Here, an automated procedure is described to identify the positions of many cryocooled crystals mounted on the same sample holder, to rapidly predict and rank their relative diffraction strengths and to collect partial X-ray diffraction data sets from as many of the crystals as desired. Subsequent hierarchical cluster analysis then allows the best combination of partial data sets, optimizing the quality of the final data set obtained. To demonstrate the general applicability of the workflow described here, we have applied it to various systems and scenarios in which many crystals of the same type are mounted on the same cryocooled sample holder. In all of the cases presented our workflow has yielded data sets that are fit for purpose.

Crystals of bacteriorhodopsin (BR) were prepared. For BR1 the initial mesh scan was carried out using a Gaussian X-ray beam of 20 µm in diameter with a flux of 3 × 1011 photons s−1. As might be expected, the protocol described here is particularly amenable to systems (i.e. thaumatin, bacteriorhodopsin, Maelstrom) that crystallize in high-symmetry space groups.

> QAQITGRPEWIWLALGTALMGLGTLYFLVKGMGVSDPDAKKFYAITTLVPAIAFTMYLSMLLGYGLTMVPFGGEQNPIYWARYADWLFTTPLLLLDLALLVDADQGTILALVGADGIMIGTGLVGALTKVYSYRFVWWAISTAAMLYILYVLFFGFTSKAESMRPEVASTFKVLRNVTVVLWSAYPVVWLIGSEGAGIVPLNIETLLFMVLDVSAKVGFGLILLRSRAIFGEAEAPEPSAGDGAAATS> ILEAAVTQSPRNKVAVTGEKV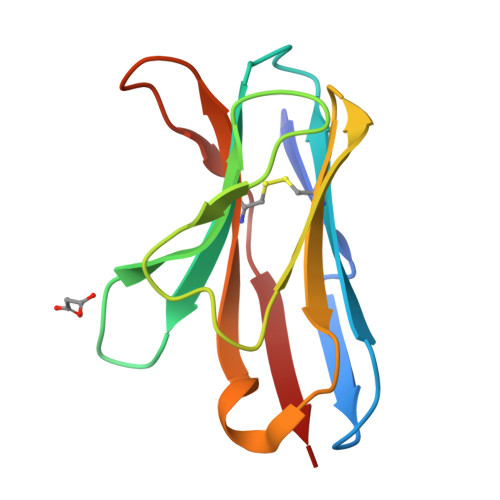TLSCQQTNNHNNMYWYRQDTGHGLRLIHYSYGVGNTEKGDIPDGYEASRPSQEQFSLILVSATPSQSSVYFCASGVGGTLYFGAGTRLSVL>MPSLQDLYAAFRRIAPYTHRTPLLTSRLLDGLLGKRLLLKAEHLQKTGSFKARGALSKALALENPKGLLAVSSGNHAQGVAYAAQVLGVKALVVMPEDASPYKKACARAYGAEVVDRGVTAKNREEVARALQEETGYALIHPFDDPLVIAGQGTAGLELLAQAGRMG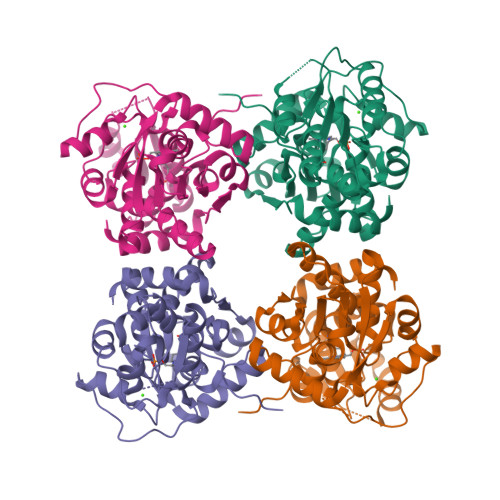VFPGAVLAPVGGGGLLAGLATAVKALSPTTLVLGVEPEAADDAKRSLEAGRILRLEAPPRTRADGVRTLSLGERTFPILRERVDGILTVSEEALLEAERLLFTRTKQVVEPTGALPLAAVLEHGARLPQTLALLLSGGNRDFSP[4x]>ASLTEIEHLVQSVCKSYRETCQLRLEDLLRQRSNIFSREEVTGYQRKSMWEMWERCAHHLTEAIQYVVEFAKRLSGFMELCQNDQIVLLKAGAMEVVLVRMCRAYNADNRTVFFEGKYGGMELFRALGCSELISSIFDFSHSLS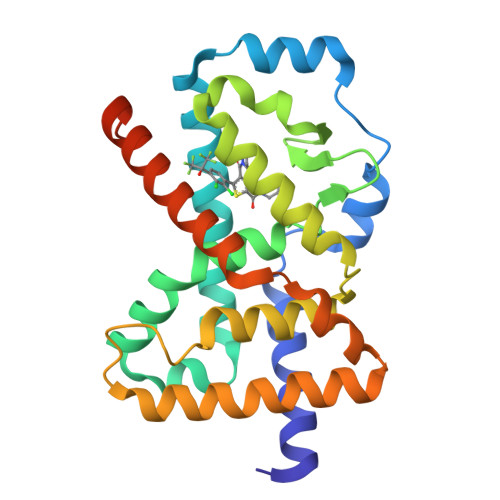ALHFSEDEIALYTALVLINAHRPGLQEKRKVEQLQYNLELAFHHHLCKTHRQSILAKLPPKGKLRSLCSQHVERLQIFQHLHPIVVQAAFPPLYKELFS[2x]>[2x]SEVEYRAEVGQNAYLPCFYTPAAPGNLVPVCWGKGACPVFECGNVVLRTD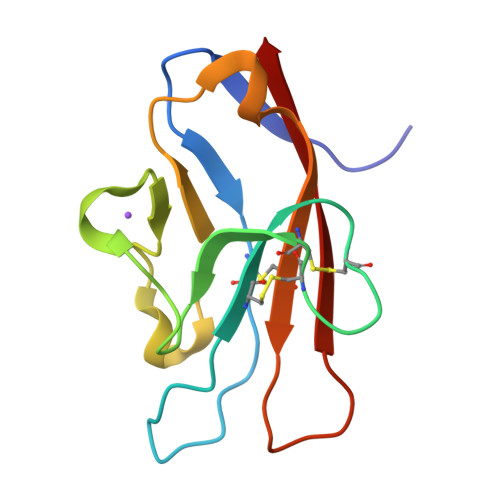ERDVNYWTSRYWLNGDFRKGDVSLTIENVTLADSGIYCCRIQIPGIMNDEKFNLKLVIK ALLOSAMIDIN | C25 H42 N4 O14 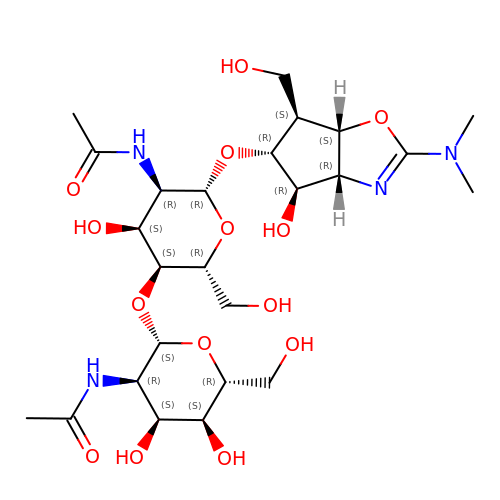| MDWNFWDBQGOKNZ-XYUDZHFQSA-N>[4x]GSSAEELLRRSREYLKKVKEEQER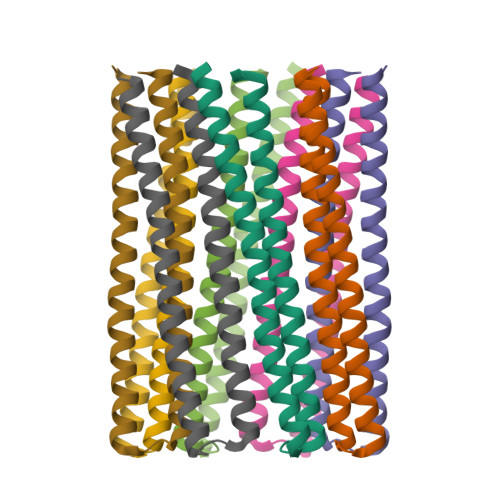KAKEFQELLKELSERSEELIRELEEKGAASEAELARMKQQHMTAYLEAQLTAWEIESKSKIALLELQQNQLNLELRHI(4S,5R)-N-{3-[(2,3-dihydroxybenzoyl)amino]propyl}-2-(2,3-dihydroxyphenyl)-N-[3-({[(4S,5R)-2-(2,3-dihydroxyphenyl)-5-methyl-4,5-dihydro-1,3-oxazol-4-yl]carbonyl}amino)propyl]-5-methyl-4,5-dihydro-1,3-oxazole-4-carboxamide 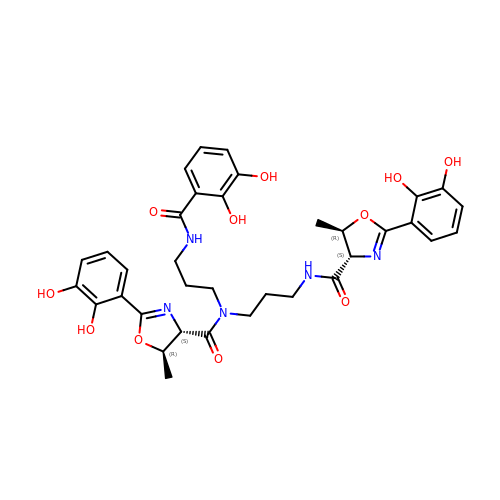| C35 H39 N5 O11 | LLMKLMMXMOTPRU-QCOILQKOSA-N> MAPVQKQFREFHDRIKLAQYDENQTLRDERDAVLTAVREGLKKVFADRGEAAPTFTPFNQGSYAMNTGVKPLEGGEYDIDVGIILNIAKDD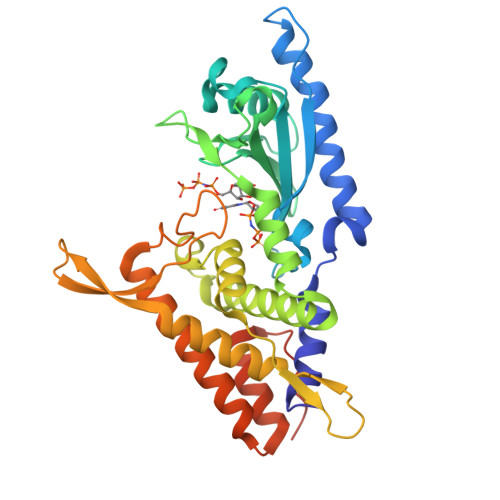HDPVEVKKWIRDALKDYGNGAEIRRSCVTVFKPGYHVDLAVYADPELSGGTLCIAKGKENSGDEHRLWQISDPQGFQDRIASKLSGDDAAQFRRCIRYLKRWRDFRFSSDGNAAPLGIGLTAAAYWWFQVSKRTDPVSQNVTYDDRDALEQFVQTMLDNFHDTWDSKDQRSYPRLTVELPVQPYNDVFEKMTGMQMESFKSKLQALLNALKTAKSRLELHDACKALADHFGSEFPVPEKDKSAVHTAPAIVGSGSSG> CGCGCGTTTTC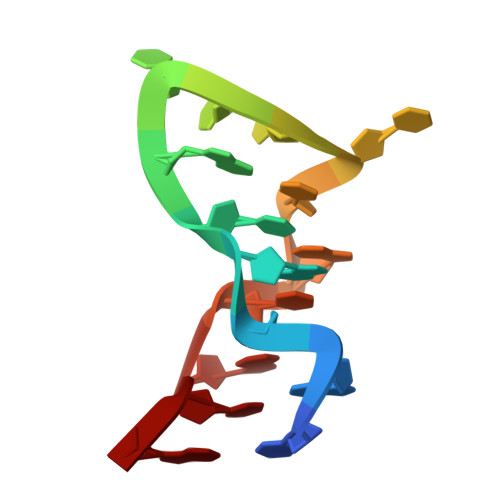GCGCG> MTHQIVTTQYGKVKGTTENGVHKWKGIPYAKPPVGQWRFKAPEPPEVWEDVLDATAYGPVCPQPSDLLSLSYTELPRQSEDCLYVNVFAPDTPSQNLPVMVWIHGGAFYLGAGSEPLYDGSKLAAQGEVIVVTLNYRLGPFGFMHLSSFDEAYSDNLGLLDQAAALKWVRENISAFGGDPDNVTVFGESAGGMSIAALLAMPAAKGLFQKAIMESGASRTMTKEQAASTAAAFLQVLGINESQLDRLHTVAAEDLLKAADQLRIAEKENIFQLFFQPALDPKTLPEEPEKSIAEGAASGIPLLIGTTRDEGYLFFTSDSDVRSQETLDAALEYSLGKPLAEKAADLYPRSLESQIHMVTDLLFWRPAVAFASAQSHYAPVWMYRFDWHPEKPPYNKAFHALELPFVFGNLDGLERMAKAEITDEVKQLSHTIQSAWITFAKT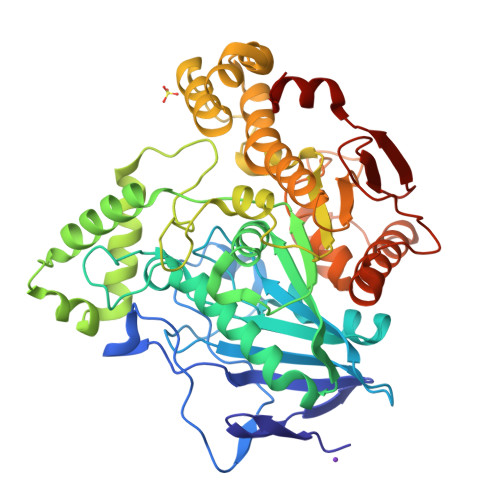GNPSTEAVNWPAYHEETRETVILDSEITIENDPESEKRQKLFPSKGE4-[4-[(4,4-dimethylpiperidin-1-yl)methyl]-3-fluoranyl-phenyl]-9-[6-(methylamino)pyrimidin-4-yl]-1,4,9-triazaspiro[5.5]undecan-2-one 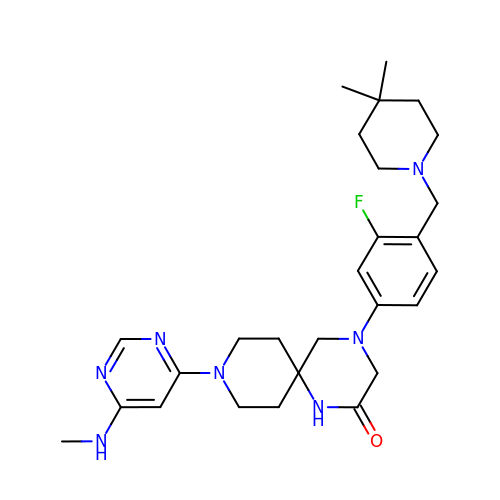| C27 H38 F N7 O | IYZMNTMLBDUPPA-UHFFFAOYSA-N> ARVTVQDAVEKIGNRFDLVLVAARRARQMQVGGKDPLVPEENDKTTVIALREIEEGLINNQILDVRERQEQQEQEAA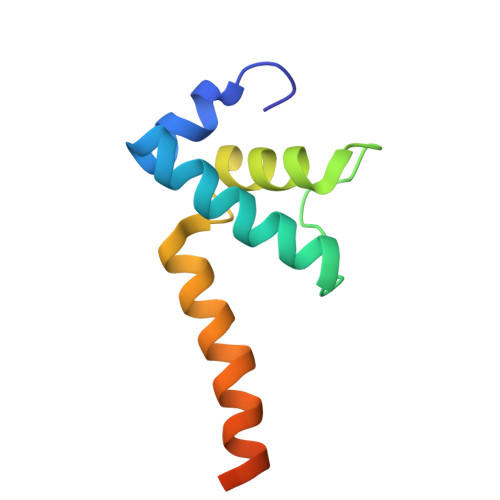ELQAVTAIAEGRR A pseudouridine kinase (PsuK) and a pseudouridine monophosphate glycosylase (PsuG) in Escherichia coli were first characterized as involved in pseudouridine degradation by catalyzing the phosphorylation of pseudouridine to pseudouridine 5′-phosphate (ΨMP) and further hydrolyzing 5′-ΨMP to produce uracil and ribose 5′-phosphate. Nevertheless, although EcPsuK and its homolog protein AtPUKI both belong to the phosphofructokinase B (PfkB) family of carbohydrate kinases, they share a low sequence identity of about 21%. Here, we solved the crystal structures of apo-EcPsuK and its binary complex with Ψ or N1-methyl-pseudouridine (m1Ψ). The structure of EcPsuK showed a homodimer conformation assembled by its β-thumb region.

To unveil the catalytic mechanism of EcPsuK for the pseudouridine substrate, we first obtained the crystal structure of apo-EcPsuK; the crystal of apo-EcPsuK was determined at 2.3Å which belonged to the space group P6322. There is one EcPsuK molecule in the asymmetric unit, which can be modeled from Arg2 to Asn308 and folded into a conformation employing the β-α unit as a basic structural motif composed of a central α/β region, and a β-stranded region protruding from the N-terminal. Furthermore, two β-strands β2 and β3 between the β1–α1, β7, and β8 between the β6–α3 extend from the central α/β structure region. These two consecutive β-strands are corporately constituting the antiparallel β-sheet in an edge-to-edge orientation (hereafter named β-thumb region). Therefore, although there is only one EcPsuK molecule in the asymmetric unit, it is a homodimer. Dimerization of EcPsuK is mainly assembled by two regions including the β-thumb region and α2 on the edge of the central β-sheet. The dimer interface adopts a face-to-face mode that looks like a butterfly with the four β-strands in the β-thumb region almost perpendicular to these elements from the adjacent asymmetric unit, which created a cross β-barrel-like fold (Sigrell et al., 1998). In detail, the β-thumb region of each monomer of the EcPsuK homodimer rigidly contacts with each other through many hydrophobic interactions, creating a hydrophobic core. Taken together, these interactions anchored the EcPsuK homodimer.

> MREKDYVVIIGSANIDVAGYSHESLNYADSNPGKIKFTPGGVGRNIAQNLALLGNKAWLLSAVGSDFYGQSLLTQTNQSGVYVDKCLIVPGENTSSYLSLLDNTGEMLVAINDMNISNAITAEYLAQHREFIQRAKVIVADCNISEEALAWILDNAANVPVFVDPVSAWKCVKVRDRLNQIHTLKPNRLEAETLSGIALSGRDDVAKVAAWFHQHGLNRLVLSMGGDGVYYSDIRGENGWSAPIKTNVINVTGAGDAMMAGLASCWVDGMPFAESVRFAQGCSSMALSCEYTNNPDLSIANVISLVENAECLN>HHHHHHEPRPNEECLQILGNAEKGAKFLSDAEIIQLVNAKHIPAYKLETLIETHERGVSIRRQLLSKKLSEPSSLQYLPYRDYNYSLVMGACCENVIGYMPIPVGVAGPLCLDEKEFQVPMATTEGCLVASTNRGCRAIGLGGGASSRVLADGMTRGPVVRLPRACDSAEVKAWLETSEGFAVIKEAFDSTSRFARLQKLHTSIAGRNLYIRFQSRSGDAMGMNMISKGTEKALSKLHEYFPEMQILAVSGNYCTDKKPAAINWIEGRGKSVVCEAVIPAKVVREVLKTTTEAMIEVNINKNLVGSAMAGSIGGYNAHAANIVTAIYIACGQDAAQNVGSSNCITLMEASGPTNEDLYISCTMPSIEIGTVGGGTNLLPQQACLQMLGVQGACKDNPGENARQLARIVCGTVMAGELSLMAALAAGHL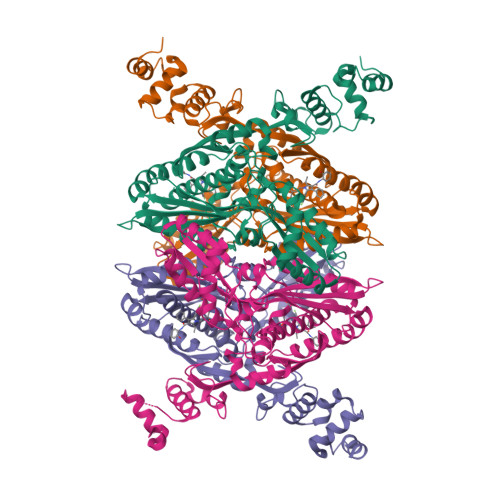VKSHMIHNRSKIN[4x]4-(1~{H}-indol-3-yl)pyrimidin-2-amine | C12 H10 N4 | 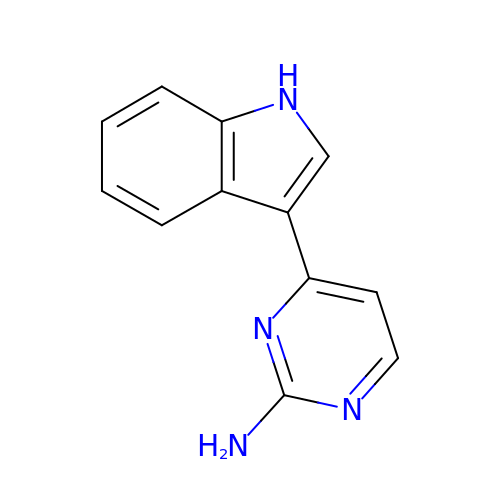QNMZWFNNJMGJPU-UHFFFAOYSA-N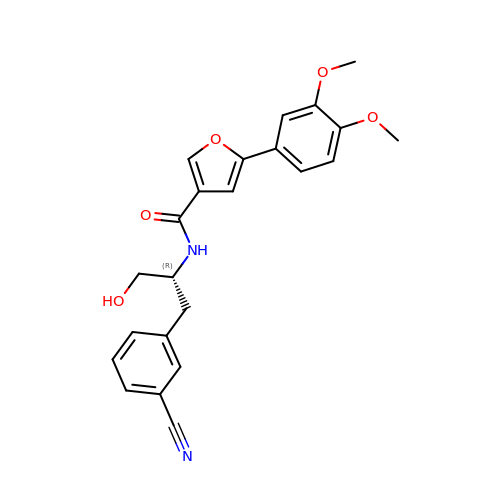N-[(2R)-1-(3-cyanophenyl)-3-hydroxypropan-2-yl]-5-(3,4-dimethoxyphenyl)furan-3-carboxamide | C23 H22 N2 O5 | WYLRQKDQMNFNCH-LJQANCHMSA-N Sodium glucose co-transporters (SGLT) harness the electrochemical gradient of sodium to drive the uphill transport of glucose across the plasma membrane. As the founding member of SGLT family transporters, SGLT1 is encoded by the SLC5A1 gene which is mainly expressed in the gastrointestinal tract and kidney. SGLT1 is essential for glucose, galactose and water uptake from the intestine and the genetic loss-of-function mutations of the human SLC5A1 gene lead to intestinal glucose galactose malabsorption. Human SGLT1 (hSGLT1) plays a key role in sugar uptake from food and its inhibitors show promise in the treatment of several diseases.

Here, we present the cryo-EM structure of the hSGLT1-MAP17 hetero-dimeric complex in the presence of the high-affinity inhibitor LX2761. We obtained a map with an averaged resolution of 3.20 Å. Therefore, the structure of the hSGLT1-MAP17 in complex with LX2761 represents the outward-open conformation. LX2761 locks the transporter in an outward-open conformation by wedging inside the substrate-binding site and the extracellular vestibule of hSGLT1. The glucose ring of LX2761 binds at the sugar substrate site of hSGLT1 and the aglycon group extends into the extracellular vestibule. In detail, at the sugar ring of LX2761, the C2-OH binds to N78 on M1, E102 on M2, and K321 on M7; C3-OH binds to the side chain of W291 on M6, and main-chain carbonyl group of F101 on M2; C4-OH interacts with side chains of T287 and W291 on M6; the methylsulfanyl group at the C5 position makes hydrophobic interactions with T460 on M11, L286, and M283 on M6. The distal amino group of amide bond on the tail interacts with D454 on M10 and its adjacent carbonyl group interacts with H525 on top of M12. MAP17 binds at the peripheral and interacts with M13 of hSGLT1. hSGLT1 shares all of the eukaryotic SGLT-specific features observed in the hSGLT2-MAP17 structure, including the extracellular shelter stabilized by three disulfide-bonds and structures packed by intracellular loops. We calculated the radius of the putative water pathway in the current SGLT1outward-open structure, showing the pathway is blocked by the intracellular gate on one side and also blocked by LX2761 on the other side. The overall structural alignment shows that half of hSGLT1, including M1, M2, M6, M7, M11, M12, and M13 are relatively stable, and we name these helices as the constant module.

> MDSSTWSPKTTAVTRPVETHELIRNAADISIIVIYFVVVMAVGLWAMFSTNRGTVGGFFLAGRSMVWWPIGASLFASNIGSGHFVGLAGTGAASGIAIGGFEWNALVLVVVLGWLFVPIYIKAGVVTMPEYLRKRFGGQRIQVYLSLLSLLLYIFTKISADIFSGAIFINLALGLNLYLAIFLLLAITALYTITGGLAAVIYTDTLQTVIMLVGSLILTGFAFHEVGGYDAFMEKYMKAIPTIVSDGNTTFQEKCYTPRADSFHIFRDPLTGDLPWPGFIFGMSILTLWYWCTDQVIVQRCLSAKNMSHVKGGCILCGYLKLMPMFIMVMPGMISRILYTEKIACVVPSECEKYCGTKVGCTNIAYPTLVVELMPNGLRGLMLSVMLASLMSSLTSIFNSASTLFTMDIYAKVRKRASEKELMIAGRLFILVLIGISIAWVPIVQSAQSGQLFDYIQSITSYLGPPIAAVFLLAIFWKRVNEPGAFWGLILGLLIGISRMITEFAYGTGSCMEPSNCPTIICGVHYLYFAIILFAISFITIVVISLLTKPIPDVHLYRLCWSLRNSKEERIDLDAEEENIQEGPKETIEIETQVPEKKKGIFRRAYDLFCGLEQHGAPKMTEEEEKAMKMKMTDTSEKPLWRTVLNVNGIILVTVAVFCHAYFA;> MSALSLLILGLLMAVPPASCQQGLGNLQPWMQGLIAVAVFLVLVAIAFAVNHFWCQEEPEPAHMILTVGNKADGVLVGTDGRYSSMAASFRSSEHENAYENVPEEEGKVRSTPM> TTNKPIVLSTWNFGLHANVEAWKVLSKGGKALDAVEKGVRLVEDDPTERSVGYGGRPDRDGRVTLDACIMDENYNIGSVACMEHIKNPISVARAVMEKKPHVMLVGDGALEFALSQGFKKENLLTAE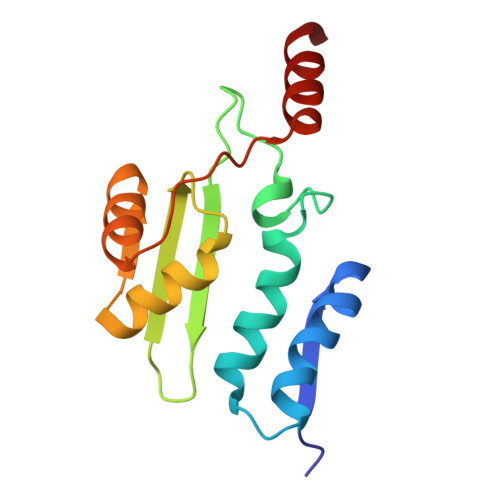SEKEWKEWLKT> DQESCKGRCTEGFNV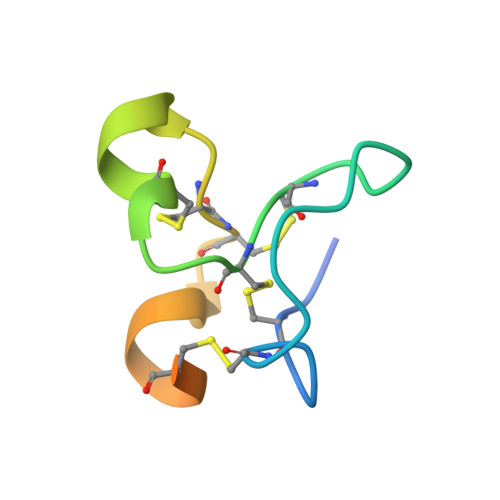DKKCQCDELCSYYQSCCTDYTAECKPQVTRGDVFTM>[2x]MKLSDLISRWIDVEPSKNAQIILRDRYFMKDLDGNYLETKWEDVARRVARVVATAELLNPSYKKNEKLDRIKEWEDIFFRVLKARLFIPNSPTLFNAGLGVKHDLLWKPIDQMTLEDYEEIYRSRNHLHMLSACFVVPVGDSIEEIFEAVKEYALITKVGGGVGSNFSELRPKGSFVAGTHGKASGPVSFMHVFNSAISVVKQGSRRRGALMGILNINHPDIEEFIDAKKENTGEAVLNFFNLSVGFPMDKKEILKLYEEDGELELSHPRSTIRKKVKIRELFRKIATNAWKSGDPGLAFLGEMNKYYPLYPHRKINSTNPCGEIGLSDYEACNLGSIDVAKFYNNGFVDLEALQELVQIAVRFL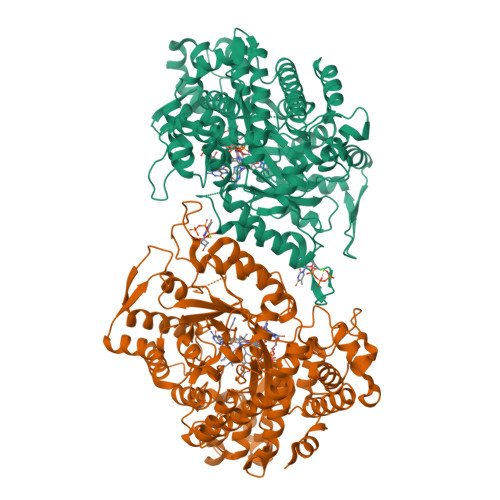DNVIDVNVFPIDKITKAVKESRRLGLGIMGFADLLYKLEIPYNSQEARDFAANLMAFIALHAHRTSYELGKEKGNFPLLEISRYRTEDNFVPFAMGMSNYDDEIREVMKMTKEFRRNVALLTIAPTGSISNIADTSSGLEPNFLLAYTRFVTKEDGTKEPLLYVNQVLREKLNPEILKRIEKELIEKGSLKDIPDVPEKIKKVFVVALDIDPMDHLLMQDAFQRYVDNNISKTINMPQSATVDDVLNVYLEALRTNVRGITVYRDGSLQTQVLTKALKT>[3x]A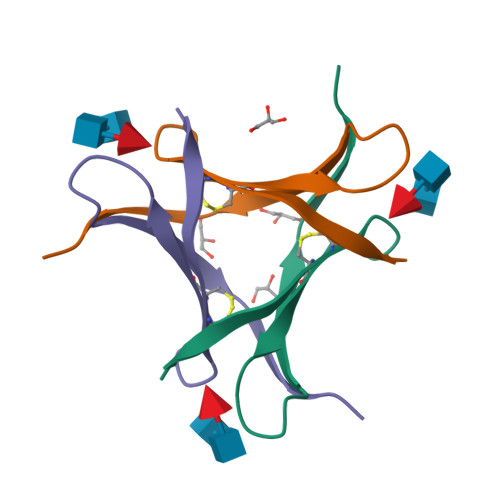PVPVTKLVCDGDTYKCTAYLDFGDGRWVAQWDTNVFHTG> GPMASMERFLSVYDEVQAFLLDQLQSKYEIDPNRARYLRIMMDTTCLGGKYFRGMTVVNVAEGFLAVTQHDEATKERILHDACVGGWMI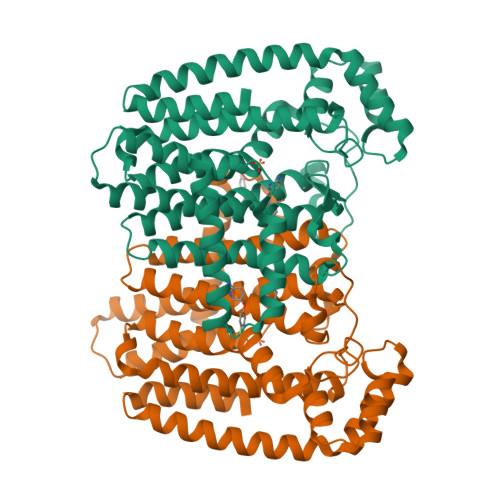EFLQAHYLVEDDIMDGSVMRRGKPCWYRFPGVTTQCAINDGIILKSWTQIMAWHYFADRPFLKDLLCLFQKVDYATAVGQMYDVTSMCDSNKLDPEVAQPMTTDFAEFTPAIYKRIVKYKTTFYTYLLPLVMGLLVSEAAASVEMNLVERVAHLIGEYFQVQDDVMDCFTPPEQLGKVGTDIEDAKCSWLAVTFLGKANAAQVAEFKANYGEKDPAKVAVVKRLYSKANLQADFAAYEAEVVREVESLIEQLKVKSPTFAESVAVVWEKTHKRKK1-oxidanylquinolin-4-one 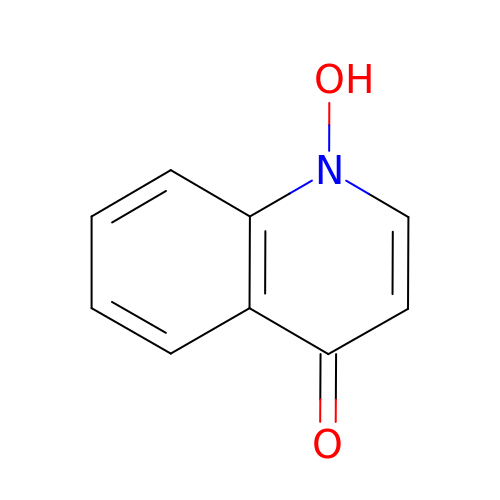| C9 H7 N O2 | AJTLULFWRGRNEZ-UHFFFAOYSA-N> MNNPAIKRIGNHITKSPEDKREYRGLELANGIKVLLISDPTTDKSSAALDVHIGSLSDPPNIAGLSHFLQHMLFLGTKKYPKENEYSQFLSEHAGSSNAFTSGEHTNYYFDVSHEHLEGALDRFAQFFLSPLFDESAKDREVNAVDSEHEKNVMNDAWRLFQLEKATGNPKHPFSKFGTGNKYTLETRPNQEGIDVRQELLK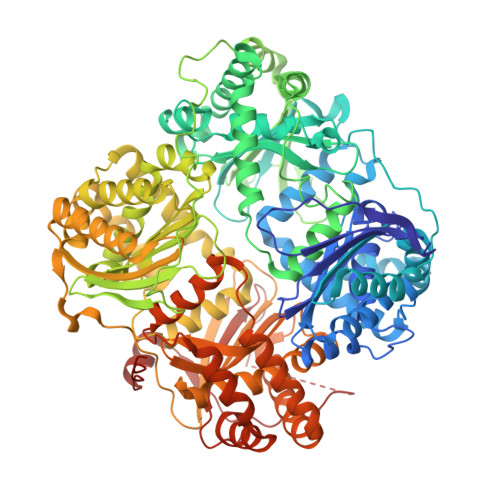FHSAYYSSNLMAVVVLGRESLDDLTNLVVKLFSEVENKNVPLPEFPEHPFQEEHLKQLYKIVPIKDIRNLYVTFPIPDLQKYYKSNPGHYLGHLIGHEGPGSLLSELKSKGWVNTLVGGQKEGARGFMFFIINVDLTEEGLLHVEDIILHMFQYIQKLRAEGPQEWVFQELKDLNAVAFRFKDKERPRGYTSKIAGILHYYPLEEVLTAEYLLEEFRPDLIEMVLDKLRPENVRVAIVSKSFEGKTDRTEEWYGTQYKQEAIPDEVIKKWQNADLNGKFKLPTKNEFIPTNFEILPLEKEATPYPALIKDTAMSKLWFKQDDKFFLPKANLNFEFFSPFAYVDPLHSNMAYLYLELLKDSLNEYAYAAELAGLSYDLQNTIYGMYLSVKGYNDKQPILLKKIIEKMATFEIDEKRFEIIKEAYMRSLNNFRAEQPHQHAMYYLRLLMTEVAWTKDELKEALDDVTLPRLKAFIPQLLSRLHIEALLHGNITKQAALGIMQMVEDTLIEHAHTKPLLPSQLVRYREVQLPDRGWFVYQQRNEVHNNSGIEIYYQTDMQSTSENMFLELFAQIISEPAFNTLRTKEQLGYIVFSGPRRANGIQGLRFIIQSEKPPHYLESRVEAFLITMEKSIEDMTEEAFQKHIQALAIRRLDKPKKLSAESAKYWGEIISQQYNFDRDNTEVAYLKTLTKEDIIKFYKEMLAVDAPRRHKVSVHVLAREMDSNPVVGEFPAQNDINLSQAPALPQPEVIQNMTEFKRGLPLFPLVKPHINFMAAKL>[5x]MEVLDLVTGPDSVTEIEAFLNPRMGQPPTPESLTEGGQYYGWSRGINLAT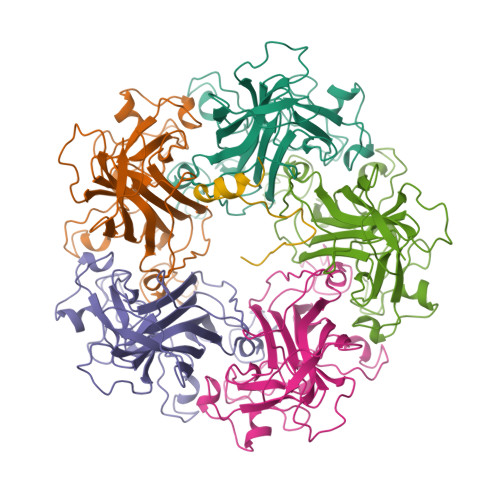SDTEDSPGNNTLPTWSMAKLQLPMLNEDLTCDTLQMWEAVSVKTEVVGSGSLLDVHGFNKPTDTVNTKGISTPVEGSQYHVFAVGGEPLDLQGLVTDARTKYKEEGVVTIKTITKKDMVNKDQVLNPISKAKLDKDGMYPVEIWHPDPAKNENTRYFGNYTGGTTTPPVLQFTNTLTTVLLDENGVGPLCKGEGLYLSCVDIMGWRVTRNYDVHHWRGLPRYFKITLRKRWVK;> GGGGGGGGAASHQRVTPDWMLPLILGLYG[(2~{R})-2-hexadecanoyloxy-3-[oxidanyl-[(2~{S},3~{S},5~{R},6~{S})-2,3,4,5,6-pentakis(oxidanyl)cyclohexyl]oxy-phosphoryl]oxy-propyl] 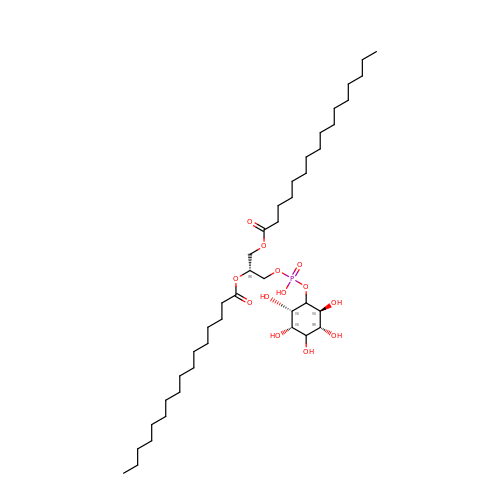hexadecanoate | C41 H79 O13 P | IBUKXRINTKQBRQ-PLWKSVIPSA-N> 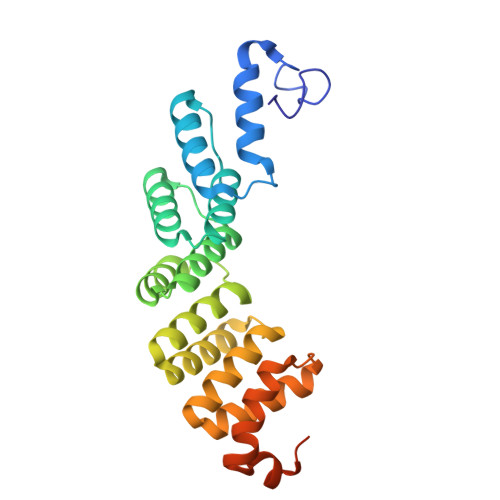MHPRLSGQGVFPRYGGGWMHQFGHVYALQQELLNAEANNWFRAMELWHTARHEGVAMNVSHYTNILRQCVPPTAWEASLMVLKQMRRENIRPDVVGVGCALAACADANRSEEVEKVFSCFSGKLKLDSICYLALIKAKMSRGGYAEALAVGREQDADGVPFLPHTYTHLLEAAEVADDGEMALELARRMSSEQWPVSDRGREALKKLSTRHHWEEVAEYKQFVAVEDHKLSLPPTLPRG> MTRVSRRGLLAVGAATGGAVVATGTARADITARSGFLWGSAGAAYQIEGGNVASDLWVVEHVQPTIFREASGDAVDAYHRVFDDIALAASLGFNAHRFSIEWSRIEPEKGQISLAAIAYYRRVLEAIRSHGMTPVVTLHHFTSPRWFAAAGGFETRDGIEPFVRYAEIVSRHLGDLFGVVATFNEPNLGGLMSWGSLSKQIRPIVQASRASAARAVNSDKFAPLVLGDFRIQTPIIIEAHERAYDVIRRETGGRTPVGLTIAVNDERAGTPDAGLDAKLEDAVLPWVRARGDFIGVQNYTYALVGKDADLPNPEGVELTQMNYPFAPEALEGAIRLVARHTDKP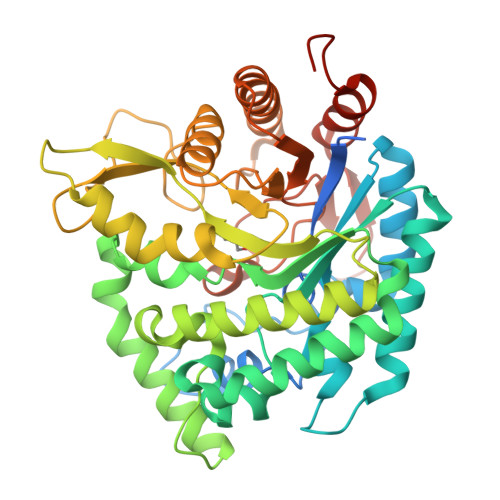IYVTENGVATEDDARRVAFIDRAVPAVFACMRDGIDVRGYIHWSFLDNWEWFAGFGPKFGLVAVDRTTFERTPKPSAAHLGRLARAGLPGDLRPLEHHHHHH>MKVLVVGNGGREHAIAWKVAQSPLVKELYVAKGNAGIWEIAKRVDISPTDVEKLAEFAKNEGVDFTIVGPEAPLVEGIVDEFEKRGLKIFGPNKEAAKLEGSKAFAKTFMKKYGIPTARYEVFTDFEKAKEYVEKVGAPIVVKADGLAAGKGAVVCETVEKAIETLDRFLNKKIFGKSSERVVIEEFLEGEEASYIVMINGDRYVPLPTSQDHKRLLDEDKGPNTGGMGAYSPTPVINEEVEKRIREEIVERVIKGLKEEGIYYRGFLYAGLMITKEGPKVLEFNVRLGDPEAQPILMRVKNDFLETLLNFYEGKDVHIKEDERYALDVVLASRGYPEKPETGKIIHGLDYLKSMEDVVV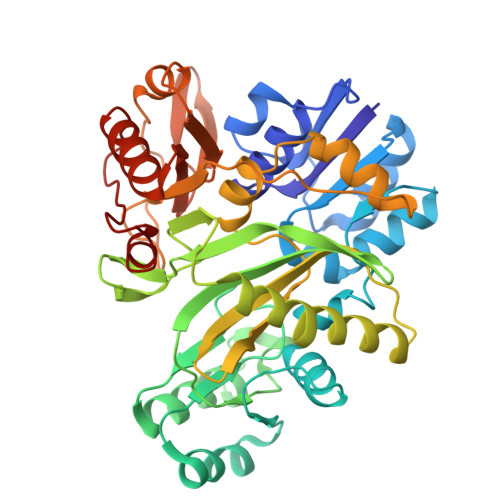FHAGTKKEGNFTVTSGGRVLNVCAYGKTLKEAKERAYEAIRYVCFEGMHYRKDIGDKAFKYLSE[2x]(1R,2S,3R,4R,5S,6S)-4-hydroxy-2,3,5,6-tetrakis(phosphonooxy)cyclohexyl trihydrogen diphosphate | C6 H18 O24 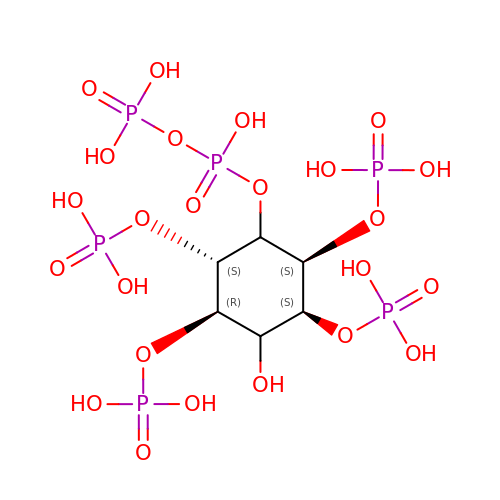P6 | FFZGWHDHUIRNPY-PTQMNWPWSA-N ArgE is a metallohydrolase in the arginine biosynthetic pathway that hydrolyzes N α-acetyl-L-ornithine to form acetate and L-ornithine (Hlaváček et al., 2014). ArgE is present in all Gram-negative and in the majority of Gram-positive bacteria. The first critical step in bacteria is the acetylation of glutamate to form N-acetyl glutamate, and the second critical and unique step is the deacetylation of N α-acetyl-L-ornithine (NAO) by ArgE to form L-ornithine. Therefore ArgE is required for cell viability, making it an attractive antibiotic target.

The two structures show a dimeric protein present in the crystals which is likely to be the biologically active form, analogous to published data on the DapE protein (Nocek al., 2014). The protein monomers consist of two catalytic domains (residues 1–179 and 305–383) and a dimerization domain (residues 180–304), with a small hinge region connecting them. The zinc-binding sites are located on the surface of the catalytic domain within the crescent-shaped substrate-binding cavity, and the zincs are coordinated by H80, E169, D112, E145 and H355 residues. The first three residues (H80, E169, D112) bind Zn1, which is present in both structures, and the last three residues (D112, E145, H355) bind Zn2, so that D112 interacts with both metal ions. The occupancy of the second zinc ion in the di-zinc structure was less than 100% and was estimated to be 80% based on visual inspection of the difference maps and refinement of metal positions. The introduction of the second zinc may be due to differences in crystallization conditions such as salt concentration and pH, but the presence of Tris buffer appears to contribute to the binding of the second zinc ion into the protein within the crystals. The Tris molecule directly interacts with five protein residues (D112, E144, E145, E169, and H355) that are involved in zinc binding and also with both zinc ions. One of the Tris oxygens is positioned between the zinc ions and may stabilize the second zinc ion in the active site. Upon examining the crystallization buffer, the Tris concentration is 100 mM, thus acting as an inhibitor at this concentration. The Zn-Zn distance determined by X-ray crystallography was observed to be 3.38 Å, nearly identical to the Zn-Zn distance of 3.39 Å determined by X-ray absorption spectroscopy.

>[4x]SNAMKNKLPPFIEIYRALIATPSISATEEALDQSNADLITLLADWFKDLGFNVEVQPVPGTRNKFNMLASTGQGAGGLLLAGHTDTVPFDDGRWTRDPFTLTEHDGKLYGLGTADMKGFFAFILDALRDVDVTKLKKPLYILATADEETSMAGARYFAETTALRPDCAIIGEPTSLQPVRAHKGHISNAIRIQGQSGHSSDPARGVNAIELMHDAIGHILQLRDNLKERYHYEAFTVPYPTLNLGHIHGGDASNRICAWCELHMDIRPLPGMTLNELNGLLNDALAPVSERWPGRLTVDELHPPIPGYECPPNHQLVEVVEKLLGAKTEVVNYCTEAPFIQTLCPTLVLGPGSINQAHQPDEYLETRFIKPTRELITQVIHHFCWH>[2x]QNNVPNTFTDPDSGITFNTWGLDEDSPQTQGGFTFG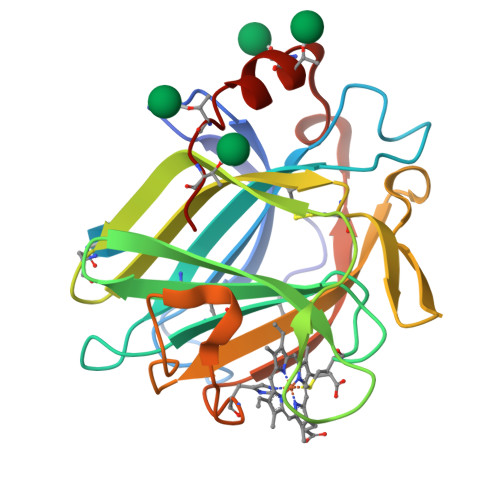VALPSDALTTDASEFIGYLKCARNDESGWCGISLGGPMTNSLLITAWPHEDTVYTSLRFATGYAMPDVYEGDAEITQVSSSVNSTHFSLIFRCKNCLQWSHGGSSGGASTSGGVLVLGWVQAFDDPGNPTCPEQITLQQHDNGMGIWGAQLNTDAASPSYTDWAAQATKTVT>[2x]MLKNVEVFWQNFLDKHELDMLMPDVWMFGDGSSEMGNRLGQLVVSGRKTATCSSLDIYKMEEEQLPKAGQYDIILDGQSQPLAIIRTTKVEIMPMNKVSESFAQAEGEGDLTLDY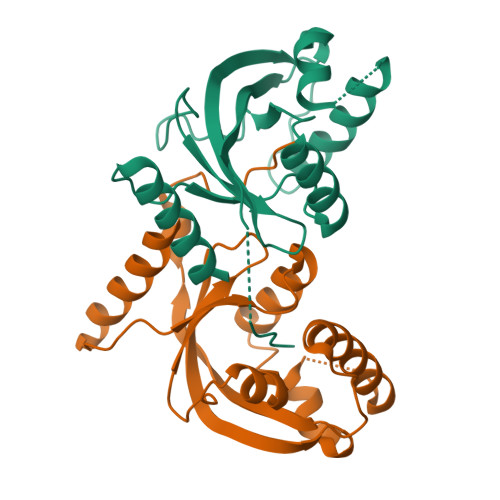WYEEHARFFKEELAPYQLQFYPDMLLVCQSFEVVDLYTEKEEGGSHHHHHH>[6x]GKLSLQDVAELIRARACQRVVVMVGAGISTPSGIPD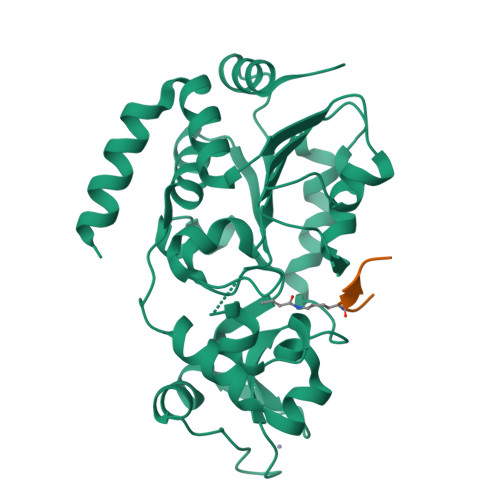FRSPGSGLYSNLQQYDLPYPEAIFELPFFFHNPKPFFTLAKELYPGNYKPNVTHYFLRLLHDKGLLLRLYTQNIDGLERVSGIPASKLVEAHGTFASATCTVCQRPFPGEDIRADVMADRVPRCPVCTGVVKPDIVFFGEPLPQRFLLHVVDFPMADLLLILGTSLEVEPFASLTEAVRSSVPRLLINRDLVGPLAWHPRSRDVAQLGDVVHGVESLVELLGWTEEMRDLVQRETGKLA;>RTKQTAR[6x]> ACRPGATRMKWYFQKPYVRRVKSDFFRFPLLSQVTKQKIDWQYHHPRSGYEAACIFGPNTLEVTNLPMGKTCQYLQERLWRFFGKFGIVEQVRVLPHERDPYQTCGTAYVCFRSRMASLRAVRLPVHLPASLHNRVLHLRHLGTDRTSDDLFYFRRQQAISNLVAIAQQLYAYLEERGPLPAHRALRLLFERSYPRLAWRQAGVSVRTCCGSWLGFFSRSPFNELFYLAREDEVARPTEVTELEADPRASRKMISNEGTEGAAETRGRKTKSKLGDTKDGTSPGLKSLTDREENAMLEKMVIFPHLLSREKLQALLLRAGRLLQMDLQNELSVHWRTDRPPLPDWTQKQIQLWQHQDPLPEELQIWSRTKDYYKIHEERFLFKLKLKKERAQAKQEMKQQRRRLE;> GADHVFNIFKDLPDHKILEDKHYPAWLFTLDKPEKTYGELAMTFLYGVGIENATLDEYLRFTRLHTKNLIKLNNMRLKKSKRSSVKPLFWDA;> GGPGRALCTPTFHGLSDGPYRRLKFSLKPIRHDYRDVLVSADLRKLAETAQELLRGKETKRRAFWEIFSKRVKASAHMLSPSLMALIAKSFDVHDRDTGIYVALATVLPEAVKRADGRSLLTLSDVFSRRLKRDSNPHLFSTLARQLPNALYQLTGKDVLRILSSLDAAGLADMLACRQVARKLLAELDELDSVDLADASAVFASQGYRNPELYSALARRAVDVKDSFDAPTVFRLLSGFSQNAVACDELLESFSTLLVSSKDQFTQHER;> KNFKTDLIRMQWPAMRDEMVRFFQSQNAIAFDKISKRHPSASLSSDASSSSSSPSANRGERRATAEEVDREEQGKLSFAEMVVGSTRSACGVLGAGRSSAVDVACKPWKRFVRKEDIQRAGYVPCIVEKYGIERRLAIHRDTLEALAFDEQHGHLSYLFQARLFRLRIGNWIEECIPTFVQADPVARRLYFVKFERHVAGKISEVDIPTTMVGLLACPAYQRGYHVELVMPTIRCQCVGAEIPPPFFVDVSRLHYSPPYTAITLQDLQHLLPADGSARFHPSYDAATQEVAWAYEVGSLPDAPLPADYVDPNFVDRKGQKMDVCFRNHFPN;> PSPSSFPHYSRRHFKRQSPRQLHQLASNLAARGCTDVVLWSSMIQRAIEVNRSPESGAADVSVAPFRFFEALGFLGAVSSLGLTDRELFLSFVPCFLRSLSALEPRHLVQLLTVYEAAGVRPRGLYVAVFNRVLKLAPSFYSHEFADFLCCLARLKIANPSFLSAFSQTLVSRLPEIAFPDACRCVGALRSLGVAQQSLFDLFDERQKKELELLPTQLLLEDFQKVLSLEFSWQAYENMIQEEFIKRTEAMIDDKDVDELADPFACLNFMKTRNLVSDKFLLALSKWCRAAVNRPATRSYKRPLAHQLVELHDLMRERNLEQNKALEQAVLRFVADDGGCKRRPREVKPLLYQRNRRYISCPDLIPDGIEPARPCAEALPDVFMERQASLVRACTPEDLARQELPFAVQAETAYRRLQRNKRFLRFVQEE;> RWRPKKSYKKRTMGLPSTKARRRWAQMRRG;> GKRYIPFRTPRNPKSKHILATPPPLFAATALDARSFVWPPLHFVERRRRLLMEKNLL;> GLWRQSIVRCADNTGVIKACIIGIRNKYGTGKIGARIRVSVRDKTPECTAPKMPKGVIVRRRKETRRKDGSYIKFDENAFVIIQKNKARGTKIKGPVPMEIRHNCKTLARWIFA;> GWSKVVNFLNKGVQRRPHRRLPGQPHHQWNMLKTQLDQLVRSDRLELTLPRAHELQQYAEELVHFAKQNTPESSLIVESMIFTPAARRKLFHELCPLYANRPFFYTRVVNQHRLRMRDAAPMAYLEFVDRPGEIRPARPVGFERKQAIWEEMQATRRGRRQWWNHAKKLGLIDEETGDVISDINALRRPSAAEWEESDSEEEKADSPSPYKMVAAPKRALEPFFVDLPPPTERYRKQRYVFKRFRP;> MTTREYEEAFLPRRLKRIKVFNTPPPSELPAFFHKRLDNAHSNPRSILKLYRQYMRKDDYPAYDWLVRCFCHLGNVFGFNSFWATKDKQVIQALPSFKFLVYDLIERKHLIEARQVPRLLYAFACLEYRSWHLLPTLLEHVEANLEKWRTPTLANMALTLALLGVGDDAPDHNQFGPPDLLSRDYTGLVSKLALEVHRRLLALQSASSSGPRKSPLHDSLGCMPFDYAGLAFALTLQGSYDLCLPSDETAKSTLALFLQRACEPLSLEQLENSGWVQFFLYQTLYCVDVEKPKREVEVKKAVPFAFQKHLHLSWLDKILINAQPQGNELLQLDVDAALKRLHITDALINCSAGRQWDEQHCWFAGHLVRSRNLALEYDYLLPLGPGRPKVSGWLACKRRMLKAFGLNVATIHQSFWSLLNLEQKDVQLTRLLAQFPPVLEAVKDEKKAYEEDRHLRFQRHARQKFETWPPEKLEI;> SQSYPKGSFHEGHINPFADVQWISRPFMKRNMPRDHHPLAKQHTSLKAVTMLDEESGNHWHVLDGKGRSVGGLAAQVVRLLQGKHRVDFTPRTAAGDSVIVVNAIHLKMAGHTWDTKVYKFDRKTHPAGPKIITAKTIMARNPAMILNLAVKRMLPPNRLRPIMYRKLFVYAGALHPHWQVPQVIVPAKTPAEVSFLPFSVERADPVQAAARIAALG;> MQIPRDVIFEVVRGFRGRSRNCIKIARVRAMKALLYSYIMRRQRQRRYRVFWIGRINAAGREWSFPYAWLATSLWRQNIWLDRKMLANLAETEPASFRALVNEGKSVYFWNPDKVRDIQDL;> VRPNQGRNDYNQVGGKKRGQGVQVLPETIRLLIETRKAATAGGPVGRQPLPKATEATGVSSWGRDRRFPITEALRLPTVAEVNAPWEPYDETANKRRSGSRPLSSSVDGCHENHDPSSDGVARGQDRLGRLDKVVLHSGDISRLRVDATVVGAVRSFKTVGDGRGFTGCSALLEGAGPFLSSFVSQQRRHLGEELLHTPVRGDPSSAQTVAAAAVRGLRRGIHHFTASTVPLPLRSSSTVPSLAEVEEMPIMELSQLAARAALLGSARGGGTRGFGLSSHPQTRRLEGVSTASGATEGSDAALSFANEVRDQATASQFPARDLIQTPLDPSQLSPPGAVLISPGFNLPSNFLIHVAEPNAVLSNQQMLDTLFRLEEREALRRKEQLLSRFGAAQAADEAMSDDEVREEDNEMTPRSMWQDDAERDTGVQRMLLLEECYINALNAAWALGVRSVALPCLGAGVGRFPVYIAARCAARGVARWMSEHRDCDAWENAESDKRADFDRIVFCTSSDVEWNALRRVIPQFLS;> GTSRRLSLFFSDPPPAYALSLHAGYKIQAALCVDRLPLVYREPRYEKRWREFKEQWEAQTKNGLTLADEITFMKFPFHFFETEEAQKKREELISKTGDAEVSELELLLSEEGFSGKRKLQRDRDAKKAAREEQSAVKSAGRGQDEKGLRSLEREPERTLYLIVRYGDSWQFPLEDRIHGQSMRSTLKRLCSEQLGSSYAPFLLGYSPFSYAKRTYPKKTKEAGILGRKIFYYRAHHIPGSENLKLPEGSPVSDFAWVTLQELPAYISPRKLAAVSAGLLLEE;> RWWTRASGMRNPVKWTRDWEVLNRKVYFAFDEREIRRSMLDAVNAHRKTASLFHRMINAVPGVAHAMSLPGPHTFFLPSDKACRDHLSPDSLHALTERVAFLEEQQRQRVGARVQVEGGVSVRGGTAAAIADRVAKTTEQLRTFVLAHLIPGEWRMKTLLLACGAGDPRRNGSLRYQDTDRELFAPVMYASRLGTGEKTKRRQTASREGVEHENAQELGRTRDEETDRSSVFLLPPPQSTDEPLPVWVQASRYAAFLPITTSTNFPRFEGTECRGNSDREEAESVENSGEYSQRRSTVGGALHLWVGGALVTKGDLRAHNGVVHMIDKPLIPVQLLAS;> WHRGTLSLLCSSCRYVVRKWHVPILGVDCNANPRHKQALSVPAPRSRGIPKHLYPFLVGKQYPRHPRWRQAFTHRSRMGKYKPQVARN;> SANPYKPKSREVFHPYVPAPEHLPPPAYTTAVLKPMQQFIPKDFYRDMRVDSLRDGVSLGSDFPWNVTHKYRFWRRRKYNIQLDDRFIRLSPVTGVDYYPRLNVFAVQWREDGQHRIRWFRAAYGLTRAMRAAENFRKTLEATGRVDN;> AISHLNPSISKGKVHYRVPNPYIPVLLLQAVPGLGKRGELKQVRRGTLRLFLAPKGLAVVASWQNIDAFYLAEKEEEERRRRAQAGR;> AKVGPSKGRGPLLAKFAPVGFKKGFGAIGLGRHTKKGFFIINTMLVPMFKVPDLSNCKLKCYVAPDTYRIVQQSFNKRE;> GILRPRERLLLNALKKEADIRYRGRRMHKRFRSWAQQRVRHYWLPQKVCVTSDPQLMDGSYIAACVQKAATLRKHDLQLWHGFSKRILELADSLTPQQMGYIFYGYGKSLFRHEELYRGLLPFVAEALPEFHSHALMTVAWALERVRVNDRAVVAQIAEEALAKKDLMRPADFIKIVNCVARMGAAPPSLAAALSAELMRVLDEKCNALLFRGAVDHVAVATLYSDPLRLYLLERFTKTAICCRPMHYQKAFQSAVAIRVLHPPVWQQLSKAVRNFYIRLSLRRIPQRARRPSPLHWDVSNALAKLGVFHRNTFQWGCFWIDIGEIDDRRQCWFVDGPSDFYSSTNEYTEANKLQHRILSELGWNIRRVRWNDWVQLGTDMDAKVEYLRKLRERPPWPAILTDGPSSSRQEMVANLRSARDVQRALKERREKNRQPHSLVMNL;> SGALQRAVREIPWKSRQDILRERERPVYAAECRGTPRREYSKNVIDGVRVKPTFNPFVKLNKAKRYVLDNWPSRNWDDWSPYRCYVRGSRRRYNIPQDLLPYKDELGEWHPPRLSARYQADVKKQYLMNNLPWVWQKDFYEGKMHFGDREPLGPKVWYRKAFREERVKEAMRKMDDLVLDYRQENRDRRRYNWFEKVVHDFAGEEIATQFIRKRKEPKL;> IATLVERSLEKHKDRLFDCGASGQPVTYKEVAEHARSISETLKAAAAYLHVPLTLPSALGRAGADGQARHTATSTEDCTGSASTLKCRGKPLNRPTIGLIVPPNSVAILAHLVGVWQCGGVGLLLPFPDPACLPFVADSTAAAAASAANAAVLFAKGGKTLHTYRPDALFQGNTGPSVYAKTVNPNSLPFLNSQNNAHNRNGVAQLWEYQAAESRCHLLVVTPEVAPMAAEVASKLSIPICVLRTSWVRKSDGTNGAEEQRAPERDLWSVRGRNKLEVKAYVPEVFHDSSRTSRNITRWQLLEVTPHECTHAAADEESIAEVAAPATHFFQGPAAHAPRAVIYSHKALSDQVIRNKDLLQLNAEDHVVILHLPFFGSHRSGTGSQASSRMLCTPKGLVAVAMPAVAAGSTLSFLSSSDKIQDSLLPLPLQLQRLQDRLPQNEKIPRQPEQRQALLPLGCDIPEKTPWRCSGTTTRGPLVPRGNQEGLQVDFTGAYENTLEVNALQMWEKIASLHEDGRNTTRSRKQRFTSRDKATPELSRQATVLAMDAETAATMVQVIATERFQMEGTNEKAHASGGSDASRFPTITSKDITRYKAAVKSLRLICICTDEGDLGASFSGRWSSSNKGGGIRIQSLLRSLQALAGPDTKILHLCSLTETGLLMVGGPLPDGSPGSRERGEKSDFGEPLQDHLSTGCKDSKTQCLDATDGEDRANFTGVVAPGIKVEIDDETDQLRVRSGHMAMGFHGRPRSTQESFDSAGLFRSSFGGSLVTNRRNDTDIIGCDRGEAEQRVELFKCVYSAAVPRLPLLHRLIASFKNSPKMESHIEGYVKKKPIAGRDWNNLHAPRKHWKKMFL;> SVVGRFRLIVPAATAKPSPAIGQTLGPLGINMMQFCKEFNARTANVRPEVPLQVTIVPLTDRSYKFSIRAPSNIWFLLRTARCPMGSESPGHQSVGNVTLKEIYHIARCKSMDWPLIGMSLRGICRSLIGTARASGIEISKEILPAYHKRDYTDVQALDSMRKDMRQRKKAAKRAAT;> YKPVIDWVKNRINARMRQYRKRSLKKKNHSKVIQRFKLTRFGWQRLRSGRNGEKENLTHKQLKRTMGYTFVSRDDLWKFRFQLPSHILRLRDAPINRNPNIRKIRRSLPSYFG;> MLWLAATHRNRVAFQLFATPREPTASKAAAAARAAAEAVARSSTVSAPFTVQKQQRLLALLAASSSVADPSADLFRVHGLPGFSGFRPSSPPHLSKLFRGRVSRHLSCRRVNHLGRNNSGRITVRFRGAGHFRRLRFVDYKRGRKDIFGTVLRLEYDPNRSAHLALLQYDDGVLSYILATEVTRPGDRVVASKHASIAPGNCLPLGNIPVSTIVHNVELRPGAGGQIVRAGGCYATVVAKDRHFVTLKLSSTEVRRFPADCWATVGQVSNAAHAERIRGKAGVSYWMGERPRTRGKAMNPVDHPHGGGTGKKGLKRPPVSKWGILCKGYKTRAKKKPLGLIVRR;> LPNPLVHLDISIGGRDAGRMVFQLFADTHPITAENFRCLCTGETGLGYWMRPRWYKSTPFHRIVPGFMCQGGDIHRGDGRGGECIYGQFFRDERFLYKHSKRGLLSMAKARRQHTNNSQFFITFDACPWLDGEHVVFGQLQSGAEVLDQIEEQGTPGGWRKRPVEIWNCGELLLNTLREIPREAPAAVRHQEMLKDLIIDATERPEKLYEPSEQVIPIPDDVYIKARRGF;> NKVRTDKKERKRAFPQRGFWKKQNFLQVKNNTVRLAFAVQGVDLLKLKRLRWGEVRKGNTGWWTDDYRSP;> IADRVRTSWTYRHSRYSGGVRFSLPRFMVTKRTYLSTKFRRPSTVTKWGNPQYTLPSNVQREMQENSAEGDTDQATSEELGGRTGKKELGRNGKSAGKTKKAADTAAQEVQHTPKYCDMLFLHQEDQQSRRR;> SRYVKVYRKVMNLQRRKTPLPWTPTFLEFSKEPSVPFPVREKLQPAPIDLSYYLNMEVGDLVEVLHGPDCGRQGVVLSISKKRNTVVVDGCNMKKSFWNPGVGASLITQEMPIHITNVALLDPVVKRPTRVKRRFMMNGECVRISKLSGSAMPEPVSTSALRQPNLYQEYLRQKALGPPLKASYARPDPLHLKILQRLARHISWGQGSPLPTAENPRVNSPEPMALRR;> RSRSKRLFVQLKSAAMTNFCYVTRKSPEKKNFRIALRKYDPGVNKHVMFYEARLPSEKNKKQITLSLQRYIRWTGKQVKLLLDKVEKAWEYGRFQKYFDNQAPLLTDRRGRAVPRYK;> SHVPYKVVRTPSGNLPVYSRVRKHGTEVTTIVRHAFGDITAMKKDLVAICEAPVRERLGTLEVKGLHVLKIKQWLRSLG;> SVASRIHFLNSRTRFQTAVHASDVAPPFLLLPLASPRPLLAYHHRFRTRNRKRGSRFHPHPLPLPPPPLSPPRSDAAHLFAGKPLAASAVSTAAGQQTLPPPLLRHLQGLFPVFRGPECDPSCGVGPAGEAAGLALLPPPSLVEPRHLEDLARRALQARGETRDAASGACKSDRLFWRELAARVEKVRDLLPIESLVRLLTILTLNGASGTVRPVKQIFQAFETQDEDTPATPANRTGLRLASETLPCVRPLPPRLLLASTREFLEDLKKLSPPATAALAATFAWSNCASSALLFALMERWAWRQPRAEPSVQTDVESEVEPLGKRREAETGVEEEAENAKKLEAVETQGHLGDFTPADFALFVSALGHLLSQQEATHVKYSRQARHLREISGKQIMAAFREQKRQKGKQTADANFENFEETKSAWHFTAAFFDGCCRFMATRAESFSLFSFASAARTLVENLDAVALVGEAAESRALAVDGEGAGSVESLGIHGISTFSSFEGSVSRSEKPHVACPTPDSVEALAKAISLFVASWDGGDKTHGRLATRAANLLLVARLLRAASQCELYIHLHRALRLEAEGSGEGKSPQKRNSGEQASGAGVDDGGRGIAVDTVGACKTLLEHISCELGLLHSELEALPLLNSTLEDADDSADEKKAVDAPTERGFVHISPDTVYVRNELLAAAGESAAAVVRLHHAKSLLQATDEVARDSQSLRKGEAENVCHLSTGARVDRVKRWMRGQQAERMQLETLGELKSEAEHLADAIDRVLRERGAAGLPTEQLADLMEVFALCVGDKRVSQTPEETSRWFRLGLGDKAEKMNQANLSSLQALSSEIVRRYAALDVNQKRRIKWATRQMDWKDPYLNHCLGRFTAAVTRQR;> YDSRWVKRLDRLRESKFYDPAPIIKEEEILEADKIHPLLKKVTPSWNSRRTGLLAYKIGMMSLWDGWGERHAVTVCQVDRCVVMDQRTLDKDGYEACVMGIGYKPIHKVTKPMLGVYIRSQIEPKSRIAEFKCSSDCLLPVGHEMSVRHFTPGQQVFVSGWSKDKGYLGVKKRWGFAGQNASHGVEAKAHSSPGSIGQSKTVNVVWRFKKMAGHAGGDPRVVNCKVFRIEAQRNLIFLKGCVPGYKGSLIKISDARGKTHHRHNRHIPLHFPTFVPEPGVSYPVTLECPDAEQDPFLYPEIAIADK;> YWPPTRKDRSKRIRLPSGKKCFVFNAKRDQDGELEPVLCFVDSQDNLLMWFNEEELLEFEKLMPRLESYYELWEEKASRTRMKEAIVAEAES;> SSGLPNTKRRIRDPFWRRSGWWRWRQQEVKAMNRSRAFRRHLFPRFTTETVSFVDAAEAEAKRFKEIVAETGRYPGQTVNFFVPKVEGAKLDPFAALPSRQKRLKLRRKAVREAEEAEKAREDADFVWRGKGGGRVWEERKANIPLGKKKLLLYCTIIKGLQITDAIDWLSSLCLHRVNYLLNLLNASRKKIHEQGGDISRVYVESYMLNIQGQIKRPQFRLRMVNLIKTWKFAVVLRFREYPMDEYFHKLFILKHVPRSLTTDMRLALAGQRVGLHAVRDWYPFLDSKTRFFHRKRLKWLDRTRQFDYCLARRVFKSKYEENCRRRKIQVLQARGASDAVIEEAN;> GNFRIKPPGARHAFPKLGTHRMVMFRRMNLLNWPPEDASPLHPIEPWGRQFFVFNAFATIDPADWCGPRGPFPRLPPLAKPAPDAATLAASPSSLLSALRETEERSATRTVMCVTDFAQRPLMFLGKDDFRALRENLPRIKEELKAFKERIQPNPVHAQYDLRRKLLVYPRQAMQRLKTGEHGGYGTRRGTIRERKT;> PPKTPRNVFFPWQVFSVHRTGAFLERRRVALKVPVNLTKFEIQSYLEKIYGARVLKVSTLIVVPRRRRDIFGPRPSMRYYRVGCTFKKAIVTLEDGVPDAVKMLRSSIELAKNPDITKHNLTYSGRVRAFKPPSAAQRWEMGESKYAWRLPIPNLLAGDEMQLNPALRIDESTTQMFPDFSKPFFHNAHFNFSWKPEEVPFQQTVKLDITPWRR;> FFYYRFHKRIGKGNFNRYLEFYQKPRGIENTLRLRYNYTPTFTAKKRSEMWKVNLVKKIAHATDAKQVLDVWTYYRHRRTKRPYHYLLALQRLVEVGGCDPTDFRFRLIARGIYRTAKRFINLPRVCVYLAKLNATGDLQDLSRFLIPQVEAYFPFQLCLLAHAFGSVRLQDKVLFAAIDEALRPHLSELPAAMLVKLTQGYAGALVHNYGLLARVSLLLQQRLSRAATGEADPLTACDEEDETGRTLSSKEPQGGSRQRETTKAAREITEAEDDCLEATEKKTVKRRHSGPLLPTLHHLLAFGRVCADLKYQDFGYLEMLSIQMQAAFRADLAVSSSRETFQRFSPFSVQELVEIFHRLKVNDVSLLLAALRHVQARMHDYPPSCVASIGFCTAQMLPCDASTVRQVHAQMLEVLQEAVPLLDLCSLGQLAAFAKKAKPRRNRSALRSSVFEAVEARVIELQGDGRTVFDVGRLLELLSLNGRRVSEEAFHILCRQAHRHLDLFEPQDFCRLARALARVKCQGSRGEQSEGLQASSLVNALARRTLRQEDEFSPRDFLSLLRSLTLAGPPDRVYAVPLKEKLRRKQVLHNYFPASQSEDAEAFEDSEQLLESDLPPSSRQTPTLRKGRLLLGPQVIRRPQQQGSPESAEGEARSEKETLEEESLSYSPVPDGEQEAEVNGNHAGKSVSVLSEGGRSRIRRRRLEEKLRIAEEEGWDLLHRRVASLRQLKGWL;> EKLYGIPHNGFWNQRRMYTEARGQTAALAAMQDPVEVLNFAGSNEMASTYLLVSCLRRVSALCDKKHAVLETVAKDERLQRLIQLISPHVDDCDARCLVDLCWAVWGFRGAPDVVEPLLNRMASVVVRRENAFTPKQLGTIAFTFSWFRGAPTDTVADFVLAECVKLLPEMEPFHVTLLFGSLRRMRRLNRDVANLMIEKLTDDIDRFTSDDVVGVLRALAANSITRGFLLRRVATLVFDNLDSFKPKQLASVLNSLTLLRFLTVENGEELFSCLSGSLSELPAASIAEILEALTILNFPRPEVVRTCLDLLAEKNGLISQGSWVRDHMIIAAHAVIQFQLYDKNPVVKPLLEELFRSRVNSSRTQHRVEEVIHALDLEKASPRVDVPPYWRAMIDQANREEQARLEHSGLQNELTLVLDSLRGKFQLQIQKNQQAGPYSVQFLDDETKICIEIDYPCCRTPHIIKARHLKQLGYHYLLVDCWQWRRLRSEAEQTVFLKQLLSGPLLEVGRL;> RLQRLIQLISPHVDDCDARCLVDLCWAVWGFRGAPDVVEPLLNRMASVVVRRENAFTPKQLGTIAFTFSWFRGAPTDTVADFVLAECVKLLPEMEPFHVTLLFGSLRRMRRLNRDVANLMIEKLTDDIDRFTSDDVVGVLRALAANSITRGFLLRRVATLVFDNLDSFKPKQLASVLNSLTLLRFLTVENGEELFSCLSGSLSELPAASIAEILEALTILNFPRPEVVRTCLDLLAEKNGLISQGSWVRDHMIIAAHAVIQFQLYDKNPVVKPLLEELFRSRVNSSRTQHRVEEVIHALDLEKASPRVDVPPYWRAMIDQANREEQARLEHSGLQNELTLVLDSLRGKFQLQIQKNQQAGPYSVQFLDDETKICIEIDYPCCRTPHIIKARHLKQLGYHYLLVDCWQWRRLRSEAEQTVFLKQLLSGPLLEVGRLEG;> RELGLGAASAIEQKASAFFSRLTDVQQRQLEKQGLLASRFYRFLVISLMEKEGTFTYYDFYVWRKGCLAYLKAAEEEMQGIVGKSARKLADLGWEKLRPSTSPEFKEMELHLKILSHFTPEELSRDTAEQFTSAAIKNIAKAAETSVKNVKNVLLGHAIALTDRTWYMRLMEMQRPIPQSVEDYLLLAETDRPYMIRLPYGEKFYNYELEEALAKKRASERHKSQRDVPRLGRKQHRIRRLFVPNARVAFDRWARIPHARLDAYGNFLYRLNQPAKGAAAVARAAEREKLRVEMSENAEFYSDAALSASRITLNNLPPGAFRRRTGMQRKSGEIHHVAPPRDPVLRELFAAAIQREKDEKRNRERRAQEDAAAAEK;> GGSYGYDAFFRGAAEVLNGSNIQLPHLPENEEQKEGKVYQLHSVRFPPQVRRLGANYFFRRQRAV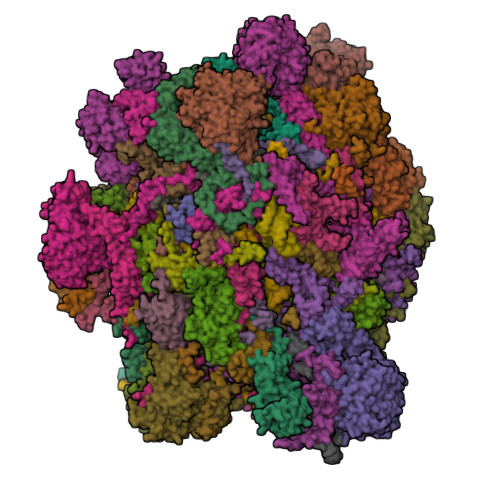PLTYYHHLVEAKPASEGSAPDGVHAQTGRGQALCFVASANPGYLQSKELENAVFESTRGFACQLILEGRGVKAYFDPEWPNLMVRLGVGVKPLALRRLAEQYATRAKIFVDKRGLLLTVHGYDKCAVGTLAMSLFNHLQANPYTMKGAHVAMHPIKKKVTR;> GIDELWKGSYLDPTIGAKQKEANAVAGDAWPACLLRMKSFEDLHKLWYICLKEKNLLMGERWAARQHKQEMKQPERLQKVRRTMRRILIVLTKREIQQQCLRAKDILAKQQKREALETRRFQLEEKMLQLEHRIRRMEPAQSLQKEAWQATLDRYRSDHEDILIQLHPLRKETTQLLAPDWRYERKYSDLPGPIRWKKQYIPALEDQYRKPIRF;> PLQPSFTPSVAFPAHKPVPLNSPLSPSVHAAPQVRRPGSVVRMNEVIRHWWSVPAVGFNSVLEVPIYRFEVFQRRAEEAGEGEASIAEEGDHPEEEEGCVVLPNDIFGLPLRPDILYRCYWFYRRAIAGWTERMQLFKWEWPGSKRKLRTQQRSGRARIGWRKAPGKYVGVKAHPLRPHDQRIKINKRLLWQGLKIMLSAKFAQGQITVVDHFNLQSHKTKHCVRHLRRLLGRKCPSALLVHEGTTDVNDNFRYATAHILAVRRENVEGINVYNLLKYRQLVITEKALLKLIYNIQTYPEKRGWLPKYATPDGKPAPAPEKVEGWDREWRQMKERERNAKFSKALLRERILKWKWSDETKGAIKVPRVDPFKGFRLARFSLHEPTMPWEKFEENYVDTDPLEDEEDGDMFDEAQALGEETQRLERLDHEELSDAAAYDDMSLTDMPLTERMHRPKRLENFKMEP;> SRSFPLGIKQTLPRHILRATGDQPSSSSSMSALAAKPPKSPCSLSVDTCKDSSPSELVVYERRDGKRWVHRHQLSLYLSHAVGLGYFRAQFEDSSVTPAAVFDCLSHLVRPPVHAARSEEDEGDEGGERRQNKQVDGAPDGDGERVTAQDLSEFMKNCVASRYRDVDVLDVVTDVLSALLIGSADLPLLVDIASSCIALSLLRPKLFTAIASRLLVLLPPAPASGSSPLDAAALSPRQAVRLVESFSHQRFRHPDVLPLLFLSLSPSLPFLSPRLACRLLHAVAGLGACAAPAETVQLLLSRVASGLGDCVGRPGCESETHCQTATGDHRMIQQTSDLPESEFLEKQIQGQKLQPQLALADLTKATHALLLLEIELEQKPLLESLLTAMAPEIFDHPVEFWSSSPAGPSLHRRLLLIRTALRHLHRDTIYNSLPTMVRQAFRRLHRIEITSPPRSPTHFVTRMSALLTRLRIAHFCYAIRGPLVFDVLERDRPIVWQCNTADRFYVNSAEKTTAVKLQERITQAMGLKVGNCEYWQWMKMKRKRTRLEYIRMQRYYILKDRRQHDPDFEGWTLPLVHHMHRRNRLHYDYYFPNYTPLSRVEY;> GVLRSLYSRVSQRVWSTLHFRVGSRGQVRTNKGFKPTAFPHLGAALFFARMSKGLTRDSVEKFVRLNVSEAQRQEIKNWPGSVVRCIENGACIPSRELQSRLEQVVGVPLTRRKKRAGNRRL;> EPKVYRQREGMIQFVFQWGIGNSFRAVSANRFRPVHAARPKEVSIHPSYFESPHPFVIWEPLNEAWEVYFYENLKKSAKPFPVKKFGIARAKREALLFLEQMKLEGKLEKPTFSSGVDGVTFDQVTGSWICRFVDEEGRCVSRGFGADFHGFEEARKLAIERQAEMKKVEASGLGPRMRLVKEK;> MASRGGTLWHLKEVVIQYSASGNSSQGLRFFFRHLLHRWKQRNPQVQVHTVENKYEAPKATFKYLGERTDSRCETPLKDLSPGQIEQILDLHRNSKGDNRFLKHGGPRTWTERRSIQGLWRPSLPSQLIALKWFRRKRPPMRLPKYSPLSLSLSIQAIRGHGRWGSEREFPRGWDQLHLKDILGSPLRSE;> MKFVHPRHWILQWKIRPGDKVVVISGKFKTIRGTVLQIDKMRNGVSVSGVKEQKRVKQEDGSFIRIPGLIHVSNVMLIDQAIDLPTRVALRVDDRGNVVRISKKSGLVIPWPNGEMIKFGDNRKSREFLKSKEERDVELRKEQNDDEERAGPKDTPAEVAVERTYDYQRDVATMQALRQMMTKYNRDFR;> NESSPLHMGAGSANWTAVARLEDFTLRGLSHPPWIHVSSRPFYGAGGGAVLAACMSSAVW;> PFKIFKASPPPAPTGRKPTGYRGNHWHKKVLYDPVYPTTKVPAALVPRYPIDWRNGGRALLIAALSKLEGASALQRRIFLRENSRESQVPQTPLSPFQTGSSASGGGAYLVSSLGRKRSYVGRIAVSLMPRHRQIADYQRVGGFCSPRCFSECSKELRRCLCAWRCTGFHEHVVQMDGMLGEYKGEVKTEKPLFSVLRRQARRNADPSEGVAFCAESAKFKSVRRAQHPAFEAFDRQGPDGPSQKPAPRKEPPLPFYSASHVPNVPRPPPPQPYTGPLKVREG;> LRHRVLPSSLPNRLFSVDNRETTRFWPPPLQKEEDERRGAFVESCLQPSGKASLLQPPQCLPRAPSHLAKLMEEEERLRLYRHLKKEERDAATLNKFGIWAGEPIADTPAAKMQPLVARTCRQTMRHLQQIEIERLDKQRNFQVPLFGPGDLMEVKYELSRSQQTFATFQGYCVEVRKKRLNSSFVLRNSYEGIGVEQRIPLYSPRIISLKVVSSCASPTQDFLLERHKPLTRDYRYKWKYNFRGRWSRRIGKHKPGIRSVEKKIRQRIVRIRKRYMGQRIEAGLPPYVWGGPYPQYGRKRSLFIRGEMYRRMLIYSFDERRRRAEKLRKRRQAVKWGVFKLRQPSVPPALTALPTYHPLYPGNLPKR;> WYTPPSKRTWSKQHNKIFTPRPLSERFSPHKLHPEFEWWRERTVQPSALFMGFPDLLALPLRGGSAYIHEMDAATLAVVLASLAHSPSAYSVSERRPPPSPSPAVSLSSSSFSPTHLPQHLDSLLALLGRQAAATAAHAPDSTLAFLFRGCAEAGVVEKNVVCTLLGRVEQRLPCMQLPECLVLLDALRPGLPEVYRHPRFVARLVAHAGLLLQFRGAESEAEDLCDLAFSLVFAANCRDAALLQTTALLLVHGKRMQSLNETAPLALARAMEAFAACRDAVNAPLLAETAAAAENGDAEGSRNTKAAELFCASPLLRAREPSVHLSPSGWLLLSLLSPVVQALHRAEKGRRKRRGFHQDGEAAGLTAEREVQNRGASRESHALTEAAARAAAAVAEETQTLKNRESSLFRGLLRCLERVDDHRESLSPGSMCKVLFAATVARAAPSRDFFPDVLKRLGDQLGACTPEDLSRALFALVKLSSVSGLDPRCQDLLPPLLGTVLQAVESSLPVADVASLARLHSAAVSALISSSETKKEEMKQLAEETSRLMHARLEEASPAHLTAFVRHWDLVPAPSGAFREALVAQAIRQLYFFDEDHLSRLLEGVTRLAASSKDETLLASVDELFRRAEEEATTEQAFFSPESCLRIFVSLVRYGEVRPEAPRNRERLVVALCNYLTGVDSVAAVSSDGASDPEELWVKEDEDLPLLFFAEDAKGFSLREDSALDRDSANESRLQALSAASYIRLLGALRELGVRGGVLLSRVAQLLHMKRYDLTDAQQEAAAEIC;> PKNLNLWGKYLRLVGRGARRGFKKWQVIPPIPVKAYGREPSAASQTGLYHDEDFNYHTKRTFSMRRTRRKIKPNVFRRTFTSSLLNVTIPNVRVTTSALHAMDDMGGFDAYILRTPPQELRSHMGERMRQVMYYYQDQPAIRDWGLPWKVFLKVASRRDPFYACYRHNLRKQQYEADLRSRVRSFSPYYLPSGHQPHAERQVFHEGAGESPPLNLWWRENRELEEAFRRRLGEAKCFERAFADSSEPLGYTKGRCRGGGGKSGRSVRRRSKTHKYRENRAF;> NAERGDADGGTSALRVTREQFHDGSRGLFRPHPFNRRFARVRKPVFPIEARNLRLMYKRKSKRRRGRGDKSNAKGIRWKHVHQQAGRYKGPRSRTFEGGKLPLYRRIPKWPDAWLARQRKVLEPLNLAKLRTFIESGRLDTRFTITQRHLNDSRCVKVKNGVSLFNVNDYPFPYKISIEVAGADQSSIDAIRRVGGEVIIVYRNRLNLRAHIKPYKFEVLPKTARPNLEMVHYLEKMRARGCVVKYVKPQWLIDEEKSLKTELAEFEAEALIAKGEAIERGDPDLRESVDDLQQRLLKRFRLRETRAAELL;> PKHLTRYLPFVPTSLVHETTSFLHDATKLRALLALIFSPCKPEASVADELASPAARLEFQQEKERYHAIRDQHTDCYRRHESAAAASMWRAIEALPSDLYEEAVQSVTFAPPYENEPPPPDPSELRPGKNASTETQAASAGQQPSAASRGSSVRTLAGPGAAGEAVSQPEHGFYHERFAFPRALMFHEMYGEQIFQSLSQLERRKLQVFMNLMHVRYPHAELKRDKPALFWLPERQVLSR;> DRFRSAVHREMIVAMTRTHLQNLLLKRFGTFKTQECRILASPAFSAVVLKAWASAVVDANLRLDGEGAMRLAYASPPPAVLSDPKVKELVASDPEAAWMLKKLSCQSVASFASLPREEEALEEVVRVKQKDNVPQPHFPSVLKMDHPQFPYEPHELEKMRDLYGVLLKWPYREQGQVASVAARRASLESKREERLRKGETEVAGQLKVTTGCSDSYVYAPSEMETGLYREHA;> MRNAIFPRIDFLRYLKKIHVSYCPTRPKTEIAKQLIMRVTSESVKKKFPHLQASWEMLAYDAPATVEVELLDGRRVRRIIDGYSKAEKKKIVDDWRFTANMEPWPEVLGPQP;> PPFRFKAPQEVRIKVPIGRIPPAVGPEIRLGKSIVAVAPHRVTAEQLEDARRVLRRVLGRSKEVHQNVHATYAVTRKPEGTKMGQGKGSIDRFVARVPAGRILFHIPQINPFHPFPEVEPNFAAFKAIAPRLPVPVVFREQNNFFQMHSVKDLIRKRQAEERENREKTARDKLGGFHTD;> TVKSLAAAEQWEPSPLTLKQHQQVVVWKKDRTCILCKKEVQGGNVEKVETACEKAWRFLSGYSRSAHVCPILPQMRILRYGELPLRDRAKFDAKLRRE;> LQIYPQRRVIGHRIEIFRGKHRRRRMVPPRIPLHPLAANTSEETASKDMNLFETYRDLQLRWKKTCRQRKKKFNIARKWRMPRNIRPLPDPSWTLVFHVNPRSGYRRGRGVCRDRRRENLQGDALEVSAEDEENRLAGKAPSNRDQEDRQRGRGAQETYFRSGAALDAAIEEENILQILARHPEKGRVEGSGRPRGADGWGRDGPLPQWMQILQRTPQEELFCVMKSNVSTQHKVTAGDLIQAEKLHRKQAGDKVVFGTVMLVGSRDWTIIGKPTVPFAKVEATVEEQTLAGETLSFFYRKSRRVSRFRRIRHCVTMLRIDRIVVDPNMTVDPPAPKPDRLLDLWANRWLYPDELDGIKRNESGEPVVSEIYDGREHQKGSYQRRGLTASYRWYPDPQSAHWRP;> TEPISHMQEKPATLRLRGLPYRTTAEDIANFFEGYSLAGPPDEAIQLHRRMDGRPTGWASVYFESEQEARRAKQDKHRSYLHGRYIEIFINFETGELEWIHQPQLSENVNRKHHGKDNRG;> GHKHSESVLQQFYNRLPVRKRFLKAIRKGTLIWDKGQVKIPPIAMQGYGLPNKLVLPHQKEFNNKLPKFKGKINQLKATRIWFQD;> ASYRRPSRASPTGQARKPHVGVRRLAAEYVWPGVVLVKQRKVIAFNVETKRRNRHFKLYPGENVKVSKVTNLVALCHGRVKFTHDVSRDVLVVNVLPERREELLREDLWRYRTEHVRSMEENRHICFLRRKAVRMFGKELVNPPTKPPLRPFYFTKYDSWENPALPDVPQLDDD;> AHKFAAPPCPNLLLLRKTIHQRLQPILFFLKNDVTMGNYVYDQHFKGVLCSPLFEGKSYKEIYAMVDRVLEDIGLSGRVKLYCEPPSLLHKMKYHVRKHWPLEKG;> IRPRKKGMRLDRRRSKKQYKHGRHVGGWNYRWLGS;> PKYDLFKPLDFLACVKSVHVAYHPGRPRSEVCRQLIHHMKSDSVRKRFPSLQASYQLLGYNAPSTIKIELINGKKHEFQAEHFSLREMQMRFDTDQFEAYLEYMKSQSVEAKP;> AVPKGKRSKHKCKQRQLIYFFDQFDGVFKRRRESFYRSFYNPPYFSKQTEQTSLPPSVLRPFRFPGFWPGRFAFKMAS;> GTQRVVQKRRHQMRILHPAQTAYVPVEQRPPPIPHSLTASSTVKRLLNNNTVAAKEAAKRINWGAYISHQRGVRWHPQGAWRVQFSRRNHERNFFVRCECYFRVGTYGFQMAKDLAIRYRQRLEKEWEELQEQWTKLDILEAEQRAKYKEKREEHLLL;> CNPQQTRRKQQYASIIGKQGLSKKQCGIFWDYYKRKCKKRRSTKKFI;> WNRNPSARYPKKGNKGCRPVCRAMRKIRKRLRTGR> MKGTIVGTWIKTLRDLYGNDVVDESLKSVGWEPDRVITPLEDIDDDEVRRIFAKVSEKTGKNVNEIWREVGRQNIKTFSEWFPSYFAGRRLVNFLMMMDEVHLQLTKMIKGATPPRLIAKPVAKDAIEMEYVSKRKMYDYFLGLIEGSSK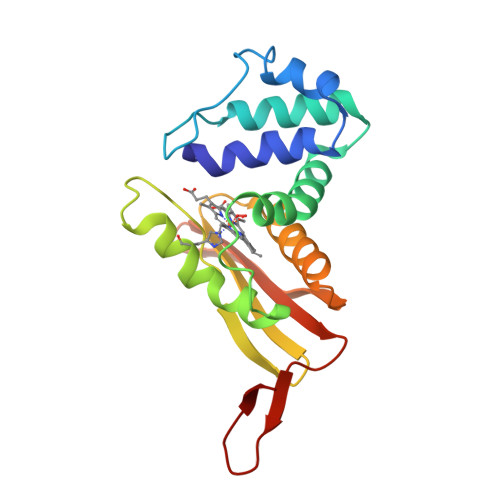FFKEEISVEEVERGEKDGFSRLKVRIKFKNPVFEYKKNVWGLVPR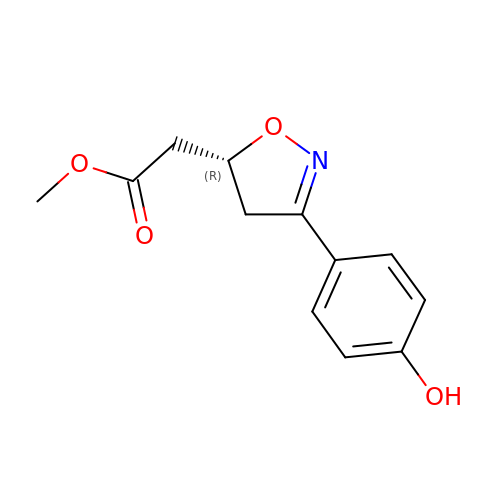3-(4-HYDROXYPHENYL)-4,5-DIHYDRO-5-ISOXAZOLE-ACETIC ACID METHYL ESTER | C12 H13 N O4 | AIXMJTYHQHQJLU-SNVBAGLBSA-N(~{E})-3-[5-(3-cyclohexyl-3,5,8,10-tetrazatricyclo[7.3.0.0^{2,6}]dodeca-1(9),2(6),4,7,11-pentaen-4-yl)furan-2-yl]prop-2-enenitrile 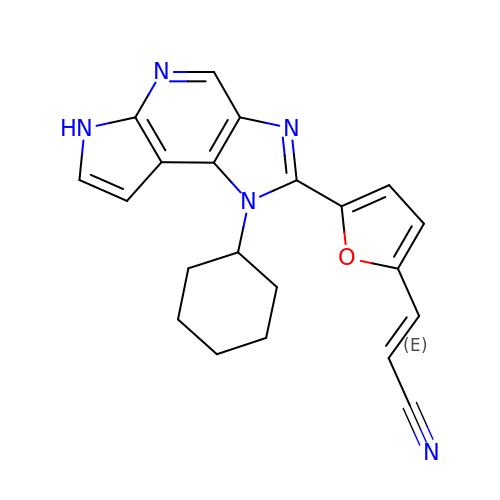| C21 H19 N5 O | UUVPPNMLZDVPOR-QPJJXVBHSA-N>[4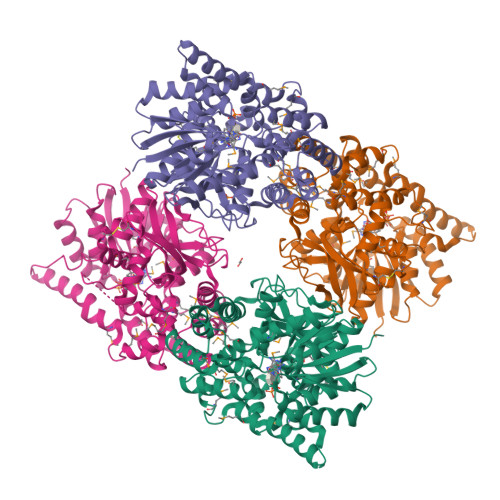x]MDKELKIVICGGGSTYTPGIVKDLLDQRQKINIKELWLYDIDEERQNKVALIVKEVIKTEAPEVVLKVTVNPKEAFTDADYIMAQMRVGGLKMRVKDEQICLKHGCVGQETCGAGGMTYGMRTIYPMVQLIDYCEEYASKKYWIVNYSNPAAIVAKATYKLRPKARIINICDMPVEIEARMAEILDCKLEDIESDYFGLNHYGWFTHVRCKGVDVTDKLKEHVRKYGYVSEASMNDALLKDPDWVHTFKNSALISSMFTDYLPNTYWQYYLMPDSIVDYMDINNTRGMQVINGREKRIFKAAEDIREGKPVDLQQFYVGVHGKFIVKVVESLIHDERSRQLVIVPNNGAIENLSDDATVEIPGYVTDRGVEPVRVGSIPRFYKGLIEQQDACEGLLVEAAIEHSYEKALMAFTMNRTIPSSLVAKKLLDDMIEANKGYWPELK>[2x]MAHHHHHHVGTNTGGVLVITDTIIVKSGQTYDGKGIKI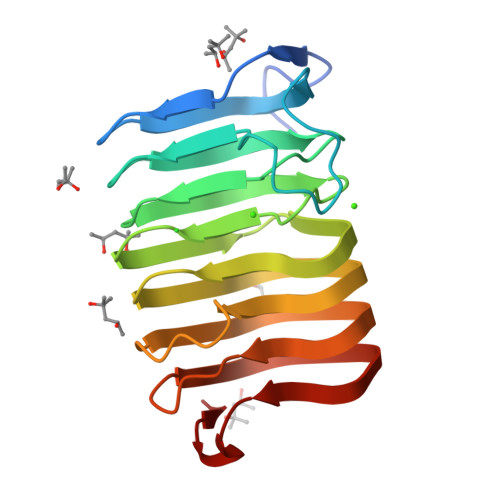IAQGMGDGSQSENQKPIFKLEKGANLKNVIIGAPGCDGIHCYGDNVVENVVWEDVGADALTVKSEGVVEVIGGSAKEAADKVFQLNAPCTFKVKNFTATNIGKLVRQNGNTTFKVVIYLEDVTLNNVKSCVAKSDSPVSELWYHNLNVNNCKTLFEFPSQSQIHQY> MEEKEILWNEAKAFIAACYQELGKAAEVKDRLADIKSEIDLTGSYVHTKEELEHGAKMAWRNSNRCIGRLFWNSLNVIDRRDVRTKEEVRDALFHHI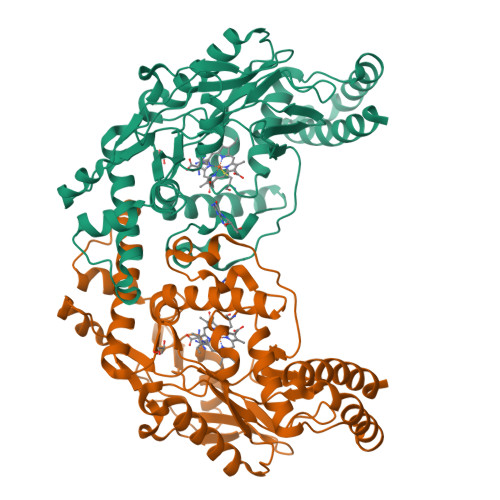ETATNNGKIRPTITIFPPEEKGEKQVEIWNHQLIRYAGYESDGERIGDPASCSLTAACEELGWRGERTDFDLLPLIFRMKGDEQPVWYELPRSLVIEVPITHPDIEAFSDLELKWYGVPIISDMKLEVGGIHYNAAPFNGWYMGTEIGARNLADEKRYDKLKKVASVIGIAADYNTDLWKDQALVELNKAVLHSYKKQGVSIVDHHTAASQFKRFEEQAEEAGRKLTGDWTWLIPPISPAATHIFHRSYDNSIVKPNYFFQDKPYE The IM component LptB2FG comprises an ATP-binding cassette (ABC) transporter, which powers the transport of LPS across the bridge. The cytoplasmic LptB dimer binds and hydrolyses ATP and the transmembrane (TM) domains of LptF and LptG create a cavity to accommodate LPS. LptB2 constitutes the cytoplasmic NBD dimer and the six TM helices of LptF and LptG (F_TM1-TM6 and G_TM1-TM6) constitute two TMDs that are arranged to form a central cavity with two surface gaps between TM1F and TM5G and TM1G and TM5F termed as lateral gates. To understand the mechanisms of how LptB2FGC recognises and acts to transport LPS, we obtained high-resolution cryo-electron microscopy (cryo-EM) structures of LptB2FGC complexed with substrate LPS or ATP analogue β-γ-imidoadenosine 5′-triphosphate (AMP-PNP).

To obtain a nucleotide-bound structure, we incubated the purified protein sfLptB2FGC with the non-hydrolysable ATP analogue AMP-PNP. Unlike the sfLptB2FGC LPS-bound structure, LptC is moved away from the lateral gate TM1G/TM5F so that the TM helix became invisible in the complex structure despite of the high resolution of 3.5 Å showing near atomic details in the cavity of the transporter. In our structures, the sfLptB2FG and sfLptB2FGC process an open cavity to accommodate LPS, while the sfLptB2FGC AMP-PNP-bound structure adopts a closed central cavity with a closed dimeric conformation of LptB. The sfLptB2FGC AMP-PNP-bound structure shows a closed dimeric conformation of LptB with clear densities for two bound AMP-PNP molecules in the ATP-binding sites at the interface of the NBDs (LptB dimer). Several residues are involved in the AMP-PNP binding site, including Y13, T44, T43, Q85, K42, E163, H195 and N38 from one LptB of the NBDs and E142, L138 and S139 from another LptB of the NBDs. In addition to the residues of LptB2, we also found that two arginine residues LptF_R292 and LptG_R301 on the cytoplasmic loop 2 of LptF and LptG extended ~9.8 and ~9.1 Å, respectively, toward the NBDs to interact with the bound AMP-PNP molecules. Interestingly these mutations showed no impact on the ATPase activity of the complex but caused cell death in the functional assays, suggesting that LptF R292 and LptG R301 residues are essential for LPS transporting but not ATP hydrolysing function of the transporter. No densities of LPS in this closed cavity was observed, suggesting a post-exporting state of LPS. Two lateral gates TM1F/TM5G and TM1G/TM5F shift into a closed conformation with their respective TM1 and TM5 helices oriented parallel to each other in close proximity, a ‘cis’ conformation. In this structure, a detergent molecule (DDM) is trapped at the lateral gate TM1F/TM5G, with hydrophobic tails trapped in the cavity while its hydrophilic head extends into the periplasm.

>[2x]MATLTAKNLAKAYKGRRVVEDVSLTVNSGEIVGLLGPNGAGKTTTFYMVVGIVPRDAGNIIIDDDDISLLPLHARARRGIGYLPQEASIFRRLSVYDNLMAVLQIRDDLSAEQREDRANELMEEFHIEHLRDSMGQSLSGGERRRVEIARALAANPKFILLDEPFAGVDPISVIDIKRIIEHLRDSGLGVLITDHNVRETLAVCERAYIVSQGHLIAHGTPTEILQDEHVKRVYLGEDFRL;> MIIIRYLVRETLKSQLAILFILLLIFFCQKLVRILGAAVDGDIPANLVLSLLGLGVPEMAQLILPLSLFLGLLMTLGKLYTESEITVMHACGLSKAVLVKAAMILAVFTAIVAAVNVMWAGPWSSRHQDEVLEEAKANPGMAALAQGQFQQATNGSSVLFIESVDGSDFKDVFLAQIRPKGNARPSVVVADSGHLTQLRDGSQVVTLNQGTRFEGTALLRDFRITDFQDYQAIIGHQAVALDPNDTDQMDMRTLWNTDTDRARAELNWRITLVVTVFMMALMVVPLSVVNPRQGRVLSMLPAMLLYLLFFLIQTSLKSNGGKGKLDPTLWMWTVNLIYLALAIVLNLWDTVFVRRLRASFSRKGAV;> MQPFGVLDRYIGKTIFTTIMMTLFMLVSLSGIIKFVDQLKKAGQGSYDALGAGMYTLLSVPKDVQIFFPMAALLGALLGLGMLAQRSELVVMQASGFTRMQVALSVMKTAIPLVLLTMAIGEWVAPQGEQMARNYRAQAMYGGSLLSTQQGLWAKDGNNFVYIERVKGDEVLGGISIYAFNENRRLQSVRYAATAKFDPEHKVWRLSQVDESDLTNPKQITGSQTVSGTWKTDLTPDKLGVVALDPDALSISGLHNYVKYLKSSGQDAGRYQLNMWSKIFQPLSVAVMMLMALSFIFGPLRSVPMGVRVVTGISFGFVFYVLDQIFGPLTLVYGIPPIIGALLPSASFFLISLWLLMRKS> MLEQPYLDLAKKVLDEGHFKPDRTHTGTYSIFG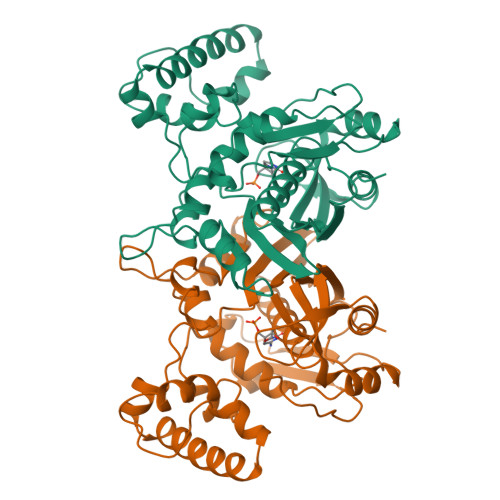HQMRFDLSKGFPLLTTKKVPFGLIKSELLWFLHGDTNIRFLLQHRNHIWDEWAFEKWVKSDEYHGPDMTDFGHRSQKDPEFAAVYHEEMAKFDDRVLHDDAFAAKYGDLGLVYGSQWRAWHTSKGDTIDQLGDVIEQIKTHPYSRRLIVSAWNPEDVPTMALPPCHTLYQFYVNDGKLSLQLYQRSADIFLGVPFDIASYALLTHLVAHECGLEVGEFIHTFGDAHLYVNHLDQIKEQLSRTPRPAPTLQLNPDKHDIFDFDMKDIKLLNYDPYPAIKAPVAV>SGEPRTRAEARPWVDEDLKDSSDLHQAEEDADEWQESEENVEHIPFSHNHYPEKEMVKRSQEFYELLNKRRSVRFISNEQVPMEVIDNVIRTAGTAPSGAHTEPWTFVVVKDPDVKHKIRKIIEEEEEINYMKRMGHRWVTDLKKLRTNWIKEYLDTAPILILIFKQV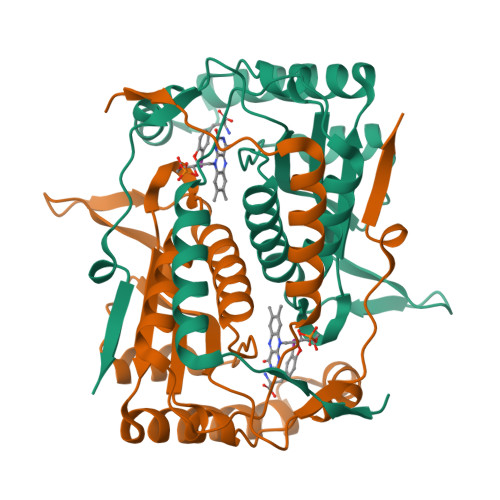HGFAANGKKKVHYYNEISVSIACGILLAALQNAGLVTVTTTPLNCGPRLRVLLGRPAHEKLLMLLPVGYPSKEATVPDLKRKPLDQIMVTVHHHHHH[6x]>[7x]SLGSDADSAGSLIQPMQIPGIIMPGLRRLTIRDLLAQGRTSSNALEYVREEVFTNNADVVA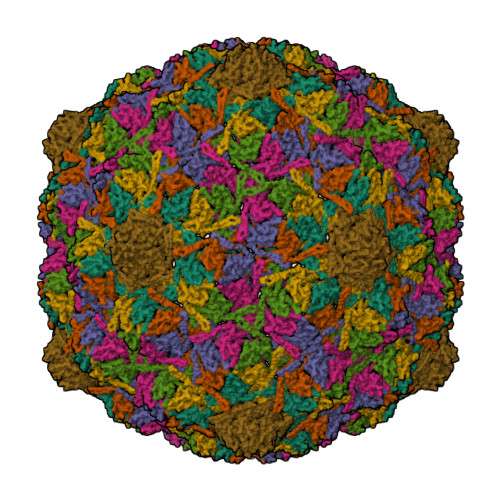EKALKPESDITFSKQTANVKTIAHWVQASRQVMDDAPMLQSYINNRLMYGLALKEEGQLLNGDGTGDNLEGLNKVATAYDTSLNATGDTRADIIAHAIYQVTESEFSASGIVLNPRDWHNIALLKDNEGRYIFGGPQAFTSNIMWGLPVVPTKAQAAGTFTVGGFDMASQVWDRMDATVEVSREDRDNFVKNMLTILCEERLALAHYRPTAIIKGTFSSGS> MGGKSNGEKKYIVGFKQGFKSCAKKEDVISEKGGKLQKCFKYVDAASATLNEKAVEELKKDPSVAYVEEDKLYRALSATS;> AKCVSYGVAQIKAPALHSQGYTGSNVKVAVLASGIDSSHPDLNVAGGASFVPSETNPFQDNNSHGTHVAGTVLAVAPSASLYAVKVLGADGSGQASWIINGIEWAIANNMDVINMSLGSPSGSAALKAAVDKAVASGVVVVAAAGNSGTSGSSSTVSYPAKY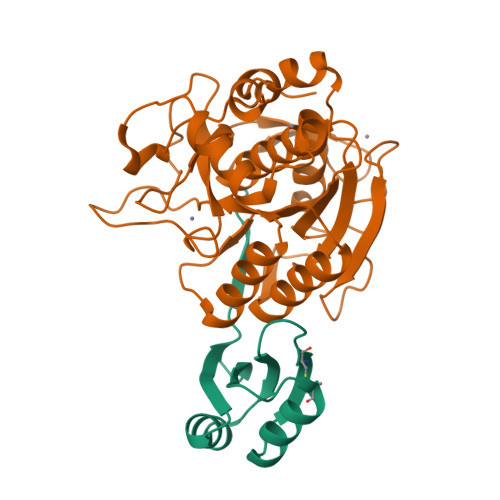PSVIAVGAVDSSNQRAPFSSVGPELDVMAPGVSICSTLPGGKYGALSGTAMASPHVAGAAALILSKHPNWTNTQVRSSLENTATKLGDSFYYGKGLINVEAAAQ> ATVQSPDGNIKIIISDEQSTPSYSISFKNKTVINNSALGFEFKQHAPFSNSFKITKVQQQSTNTQWQQPWGERQTVVDQHNEVTVTFAKPQPQGGTYSVRFKAFDSGVGFRYEVPKQAGLNNIEITKELTEFAVNNSHTATAWWIPARGWNRYEYVYNTTPLNDAALVHTPFTFKNQDGVHISIHEAALVDYAAMVLNQRRPGVFQADLTPWSSGVAVKKQGAFNTPWRTIQIGEKAVDLVNSDIILNLNEPNKLGDVSWVKPGKYIGIWWGMHINTHTWGSGDKHGATTKNTKYYMDFAAKYGFDGVLVEGWNTGWDGDWFFNGDVFSFTQPYDDFDIAALTKYSKQTGVQLIGHHETSGNVSNYRKQMADAFALYEKSNVSQVKTGYVADGGNIKRIDKNGIARHEWHDGQFMVNEYLHNVKLAAKHKISINTHEPIKDTGLRRTYPNWITREGARGQQFNAWGTPPNPPEHISMLAFTRMLAGPMDFTPGIFDLSFNGLGANTNRPQTTLAKQLALYVVLYSPIQMAADLPKNYLAKPDAFQFIQDVPTDWQQSIALDGAVGDFIVFARKERKRDKYTGNDWYLGAVTDEQARTIEISLDFLDNGKQFEAHIYKDGKNAEWKNNPY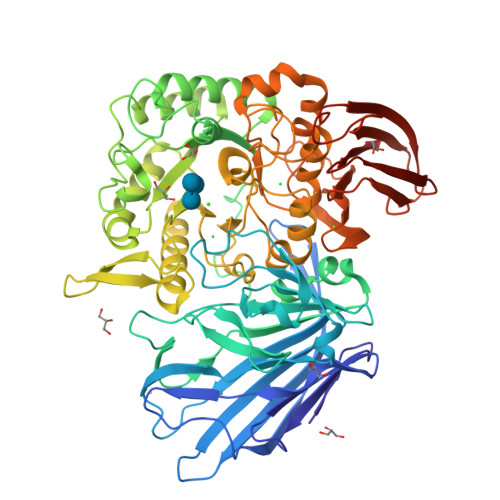DLTIEKRLVTASDKLTLKLATSGGTAIRFKALLEHHHHHH> DVPQWEV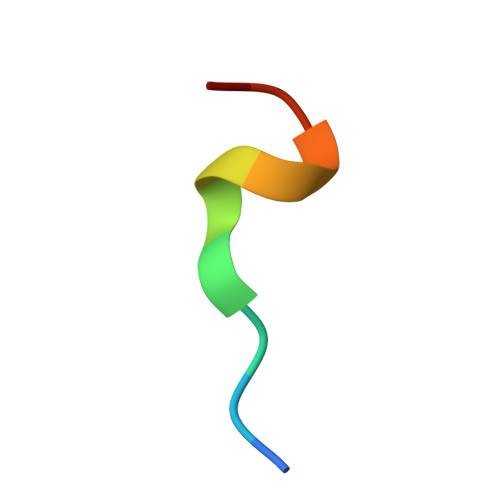FFKR>[2x]MASPNPLAFEAATAAHEVAASYVTEHKPRKNDNINFANFNQDFSCVSVGYSNGYKIYNCEPFGQCYSKSDGSIGIVEMLFSSSLLAIVGMGEQHSLSPRRLKIINTKRQTTICELTFPGAILAVKLNRERLVVLLEETIYIYDINNMRLLHTIETPSNPNG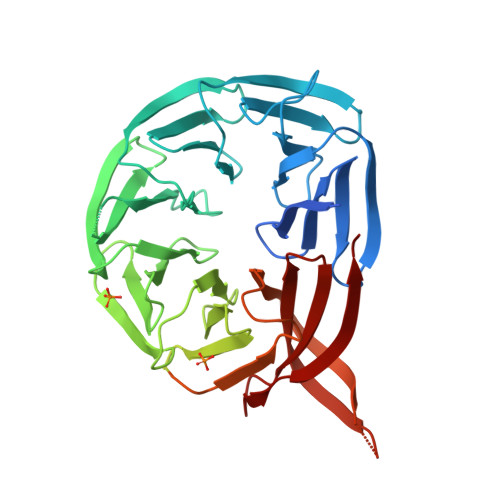LIALSPSSENNYLAYPSPQKLAPNPQTEVTLHSNPQTVRNGDVIIFDAKTLQPTSVIEAHRTSLAAIALSKDGLLLATASDKGTIIRVFSVATGIKLYQFRRGTYPTKIYSLAFSPDNRFVIASSATETVHIFRLGEEEAANTIKSANKKARLTKAQVPNPLETSPDIYPHNQHTSSDEDEELNEDEEDLDGDEDEDLEDDAHVPVSLQRGRSSSSTGSFHSSESMTDKLKEPLVDNSRKSVARMLRRTSQSLGRKAAEKMGTYLPPKFSSILEPNRHFASLKVPASKETKTVVGVGSKIWDDLIPSVYLKDDANSITETSEDLVNKKLVHIMVITSEGFFYKFGLDPERGGDCVLLHQQSLFG> MAAAAWLQVLPVILLLLGAHPSPLSFFSAGPATVAAADRSKWHIPIPSGKNYFSFGKILFRNTTIFLKFDGEPCDLSLNITWYLKSADCYNEIYNFKAEEVELYLEKLKEKRGLSGKYQTSSKLFQNCSELFKTQTFSGDFMHRLPLLGEKQEAKENGTNLTFIGDKTAMHEPLQTWQDAPYIFIVHIGISSSKESSKENSLSNLFTMTVEVKGPYEYLTLEDYPLMIFFMVMCIVYVLFGVLWLAWSACYWRDLLRIQFWIGAVIFLGMLEKAVFYAEFQNIRYKGESVQGALILAELLSAVKRSLARTLVIIVSLGYGIVKPRLGVTLHKVVVAGALYLLFSGMEGVLRVTGAQTDLASLAFIPLAFLDTALCWWIFISLTQTMKLLKLRRNIVKLSLYRHFTNTLILAVAASIVFIIWTTMKFRIVTCQSDWRELWVDDAIWRLLFSMILFVIMVLWRPSANNQRFAFSPLSEEEEEDEQKEPMLKESFEGMKMRSTKQEPNGNSKVNKAQEDDLKWVEENVPSSVTDVALPALLDSDEERMITHFERSKMESNSLEVLFQ

TMEM87s are eukaryotic transmembrane proteins with two members (TMEM87A and TMEM87B) in humans. TMEM87s have proposed roles in protein transport to and from the Golgi, as mechanosensitive ion channels, and in developmental signaling. TMEM87A consists of a Golgi-dynamics (GOLD) domain atop a membrane-spanning seven-transmembrane helix domain with a large cavity open to solution and the membrane outer leaflet. We propose TMEM87A and structurally homologous GOST proteins could serve a common role in trafficking membrane-associated cargo.

Full-length human TMEM87A was expressed and purified from Sf9 insect cells and reconstituted into lipid nanodiscs composed of MSP1D1 and a mixture of DOPE, POPS, and POPC lipids. Cryo-EM was used to determine the structure of TMEM87A to a nominal resolution of 4.7 Å, with better resolved regions reaching ~4.3 Å in the core of the protein. About 37 N-terminal residues (amino acids 1–37), 88 C-terminal residues (475-555), and 36 residues in loops within the extracellular domain (145–173, 192–198) were not resolved in the cryo-EM map and are unmodeled. The second, between C89 and C431, tethers the bottom of the extracellular domain to the top of the 7TM domain in the H6–H7 linker, perhaps constraining their relative movement. In TMEM87A, helix 8 turns back towards the center of the protein and packs against the bottom of the transmembrane domain. The position of helix 8 in TMEM87A would sterically clash with putative G-protein or arrestin binding through interfaces analogous to those observed in GPCR structures. In TMEM87A, this cavity measures approximately 8,637 Å as compared to 12,350 Å for the WLS cavity. It is funnel-shaped, presenting a large opening to the extracellular side near the GOLD domain and tapering closed near the intracellular surface above helix 8. H5 and H6 are splayed apart to open a large ‘slot’ between the cavity and the upper leaflet of the bilayer. Density within the membrane exposed portion of the hydrophobic cavity is consistent with a bound phospholipid. A partial lipid is modeled based on density, chemical environment, and relationship to WLS, but we note this assignment is speculative given the relatively low resolution of the reconstruction.>MGAPVLPAAFGFLASARTGGGRAPGPVFATRGSHTDIDTPQGERSLAATLVHAPSVAPDRAVARSLTGAPTTAVLAGEIYNRDELLSVLPAGPAPEGDAELVLRLLERYDLHAFRLVNGRFATV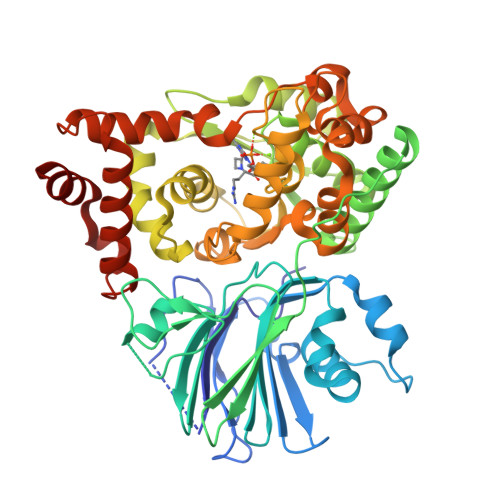VRTGDRVLLATDHAGSVPLYTCVAPGEVRASTEAKALAAHRDPKGFPLADARRVAGLTGVYQVPAGAVMDIDLGSGTAVTHRTWTPGLSRRILPEGEAVAAVRAALEKAVAQRVTPGDTPLVVLSGGIDSSGVAACAHRAAGELDTVSMGTDTSNEFREARAVVDHLRTRHREITIPTTELLAQLPYAVWASESVDPDIIEYLLPLTALYRALDGPERRILTGYGADIPLGGMHREDRLPALDTVLAHDMATFDGLNEMSPVLSTLAGHWTTHPYWDREVLDLLVSLEAGLKRRHGRDKWVLRAAMADALPAETVNRPKLGVHEGSGTTSSFSRLLLDHGVAEDRVHEAKRQVVRELFDLTVGGGRHPSEVDTDDVVRSVADRTARGAA[2x]>NGMLYPQSNDSRIVFPLDGVWDFRTAGEDSYPAEWADAPLPEPLPMAVPGSYNDQNDELNLRAHYGWVVYQRSFAVPSRLVAGQRMILRFDAATHAADVYLNGQLLGSHFGGFLPFEFDVTSALHAGENLLTVAVDNRIGSSTLPVGNDAGTAFMGSDNANVPAVAEAKKHARRQNLPNFDFFNFAGLNRHVELYTTPADAYIADIAITTERLDHIAGDACTAANALIAYDVTFGGDFPSNPTDPNTPIQPSDPAINHADSSESAESDIQRATTYGRQVRISILDGEGTVVAGVTADIERSGDGTAKASGEIAIRDAKLWNPGAAYLYTAVAELLPEGGAESSSRIIDAYRQTFGIRTVEVSGTTFLINGKPFYFKGFGKHEDSYFHGRGTDDVLNVKDVSLIHWLHANSFRTSHYPYAESMYDLCDREGIVIIDEVPAVGMSWLQYANPLVAERHREAIRGMIARDKNHPCIVMWSIANEPGLDGDGERPRQAYDYFRPLYELAHASDPQNRPVTLVCCQNDY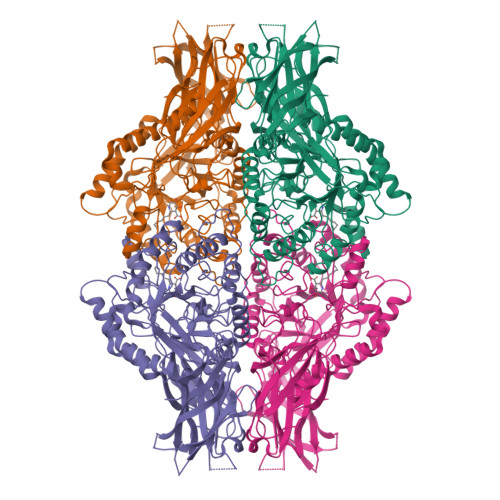TTDITERTMDVVCINRYYGWYNLSGDLDAACHALNIELDFWENIGKPVMFTEYGADTIEGIHGTHGEMFSEEFQRDYYARINAEIDKRPWFIGEQLWNFADFATFQGIIRVEGNRKGILTRDRQPKMAAHWLRERWAGIPDYGYKG[4x]>MKITNPVLKGFNPDPSICRAGEDYYMAVSTFEWFPGVQIYHSKDLIHWRLAARPLQKTSQLDMKGNPDSGGVWAPCLSYADGQFWLIYSDIKVVDGPFKDGHNYLVTADAVDGEWSDPVRLNSSGFDPSLFHDPSGKKYVLNMLWDHREKHHSFAGIALQEYSVSEKKLVGERKVIFKGTPIKLTQAPHLYYINDVYYLLTAEGGTRYEHAATIARSSRIDGPYEVHPDNPILTAFHAPSHPLQKCGHASIVQTHTNEWYLAHLTGRPIHSSKESIFQQRGWCPLGRETAIQKLEWKDGWPYVVGGKEGLLEVEAPAMSVKEFSPTYHIVDEFKDSSLNRHFQTLRIPFTDQIGSVTENPHHLRLYGQESLTSKFTQAFVARRWQSFYFEAETAVSFFPKNFQQAAGLVNYYNTENWTALQVTYDDALGRILELSVCENLAFSQPLIKKIIIPDEIPYVYLKVTVQRETYTYSYSFDQQEWEKIDVPLESTHLSDDFIRGGGYFTGAFVGMQCQDTSGERLPADFKYFRYEETTEHHHHHH[2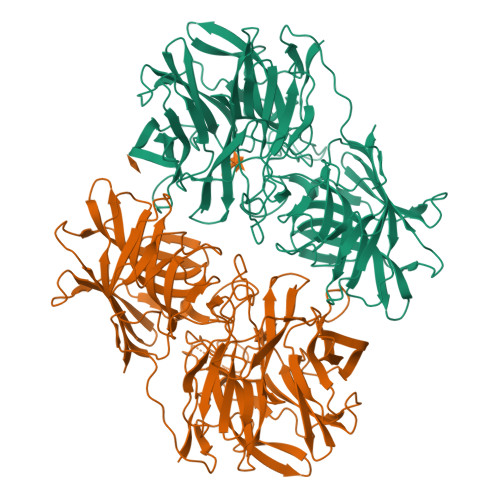x]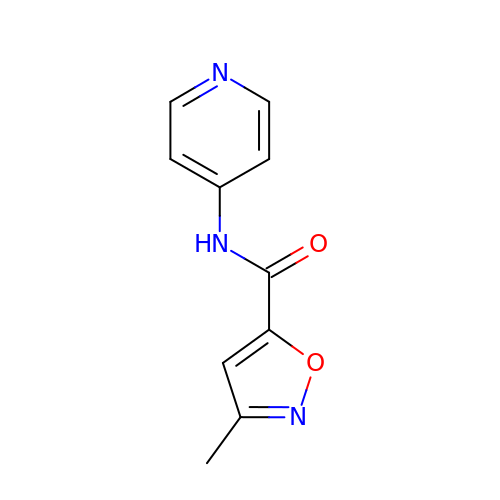3-methyl-N-(pyridin-4-yl)-1,2-oxazole-5-carboxamide | C10 H9 N3 O2 | HPNYMQLDUOKPSU-UHFFFAOYSA-N(N5,C4A)-(ALPHA-HYDROXY-PROPANO)-3,4,4A,5-TETRAHYDRO-FLAVIN-ADENINE DINUCLEOTIDE | C30 H43 N9 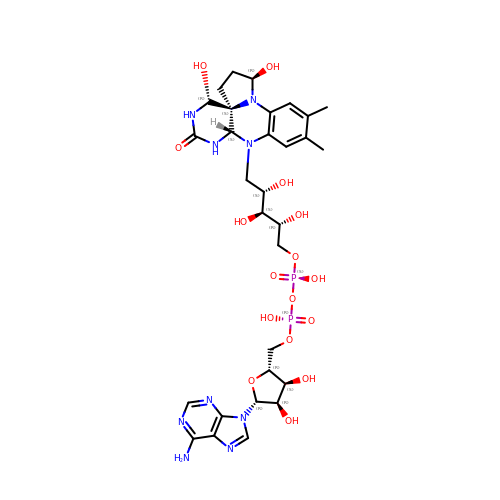O16 P2 | JIPQJEPHOHUOJG-VWUOBWNNSA-N> GSMPKPINVRVTTMDAELEFAIQPNTTGKQLFDQVVKTVGLREVWFFGLQYVDSKGYSTWLKLNKKVTQQDVKKENPLQFKFRAKFFPEDVSEELIQEITQRLFFLQVKEAILNDEIYCPPETAVLLASYAVQAKYGDYNKEIHKPGYLANDRLLPQRVLEQHKLTKEQWEERIQNWHEEHRGMLREDSMMEYLKIAQDLEMYGVNYFEIKNKKGTELWLGVDALGLNIYEHDDKLTPKIGFPWSEIRNISFNDKKFVIKPIDKKAPDFVFYAPRLRINKRILALCMGNHELYMRRRKPDTIEVQQMKAQARVDSSGRI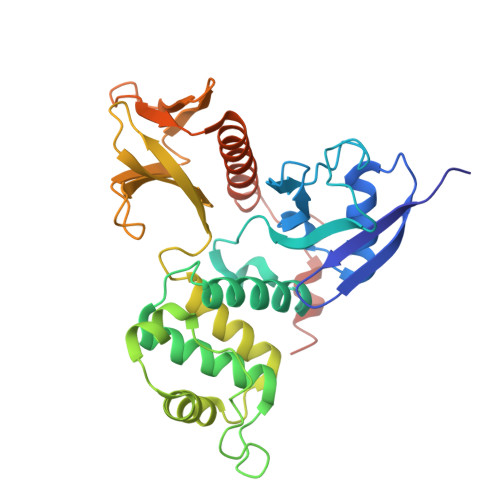VTD>[2x]GPLVLIGSGLSSEQQKMLSELAVILKAKKYTEFDSTVTHVVVPGDAVQSTLKCMLGILNGCWILKFEWVKACLRRKVCEQEEKYEIPEGPRRSRLNREQLLPKLFDGCYFYLWGTFK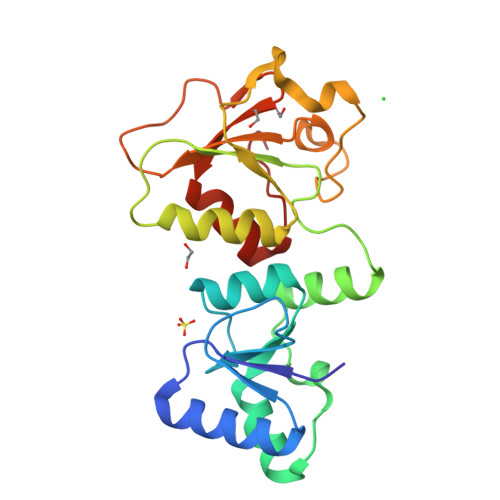HHPKDNLIKLVTAGGGQILSRKPKPDSDVTQTINTVAYHARPDSDQRFCTQYIIYEDLCNYHPERVRQGKVWKAPSSWFIDCVMSFELLPLDS> MTQAKAKHADVPVNLYRPNAPFIGKVISNEPLVKEGGIGIVQHIKFDLTGGNLKYIEG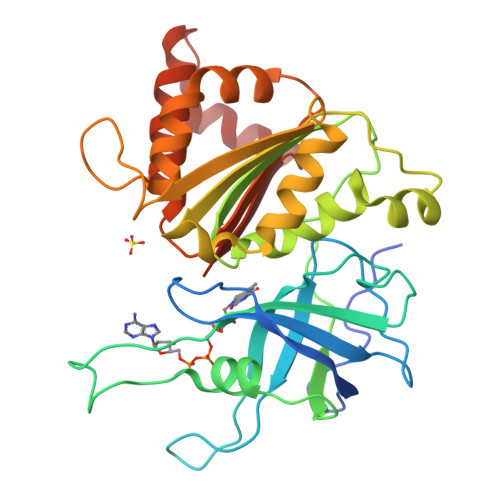QSIGIIPPGVDKNGKPESLRLYSIASTRHGDDVDDKTISLCVRQLEYKHPESGETVYGVCSTYLTHIEPGSEVKITGPVGKEMLLPDDPEANVIMLATGTGIAPMRTYLWRMFKDAERAANPEYQFKGFSWLVFGVPTTPNILYKEELEEIQQKYPDNFRLTYAISREQKNPQGGRMYIQDRVAEHADQLWQLIKNQKTHTYICGLRGMEEGIDAALSAAAAKEGVTWSDYQKDLKKAGRWHVETY> MGSSHHHHHHSQDPNSMTTLTRQDLNFGQVVADVLCEFLEVAVHLILYVREVYPVGIFQKRKKYNVPVQMSCHPELNQYIQDTLHCVKPLLEKNDVEKVVVVILDKEHRPVEKFVFEITQPPLLSISSDSLLSHVEQLLAAFILKISVCDAVLDHNPPGCTFTVLVHTREAATRNMEKIQVIKDFPWILADEQDVHMHDPRLIPLKTMTSDILKMQ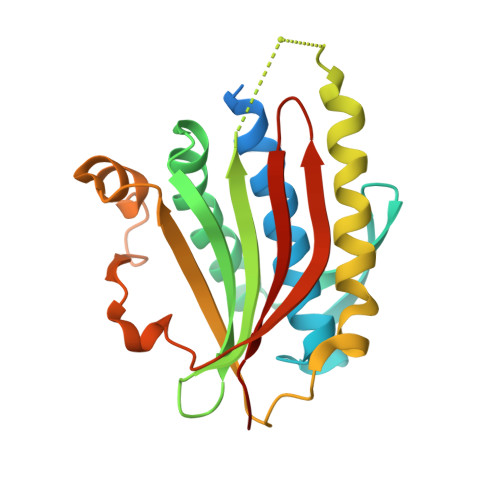LYVEERAHKGS>TDLPRPSISAEPGTVIPLGSHVTFVCRGPVGVQTFRLERERNYLYSDTEDVSQTSPSESEARFRIDSVNAGNAGLFRCIYYKSRKWSEQSDYLELVVK[2x];>VTAKELAEKAGAAAGLKAGDIHGMKIV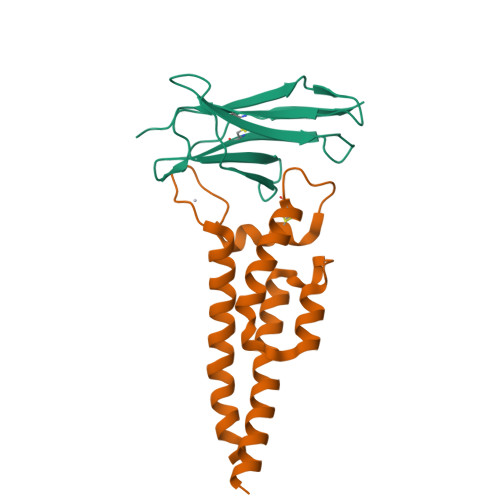IEGLKALKVDTLKSGIFNSFVQNSHYTEVTGLAIAIDTEMNEVCSATYIGIHPICVVREKLGVIPKAGGTMVKQKDAITNVLKQALEKATQSAEALSETTAEDVAAKLTAQKTGAINT[2x]> GPHMERIEGRVAA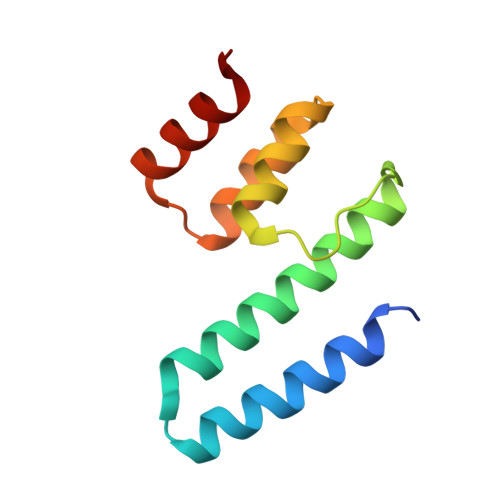LQTAADAFYKAKNEFAAKATEDQMRLLRLQRRLEDELGGQFLDLSLHDTVTTLILGGHNKRAEQLARDFRIPDKRLWWLKLTALAD ETHYL 4-[(4-METHYLPYRIDIN-2-YL)AMINO]PIPERIDINE-1-CARBOXYLATE 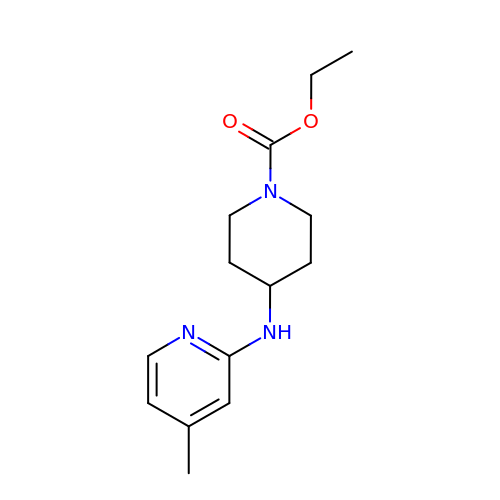| C14 H21 N3 O2 | LNRMJBWADUSJTA-UHFFFAOYSA-N>PNFSGNWKIIRSENFEELLKVLGVNVMLRKIEVAAASKPAVEIKQEGDTFYIKTSTT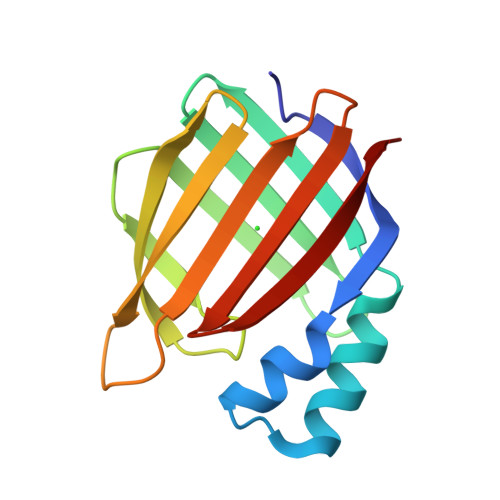VRTTEINFKVGEEFEEQTVDGRPCKSLVKWESENKMVCEQKLLKGEGPKTSWTLELTNDGELILTMTADDVVCTKVYVRE[2x]> MNYEEVIKKYRGEENFDHAAYDWRLHSGVTPVKDQKNCGSAWAFSSIGSVESQYAIRKNKLITLSEQELVDCSFKNYGCNGGLINNAFEDMIELGGICPDGDY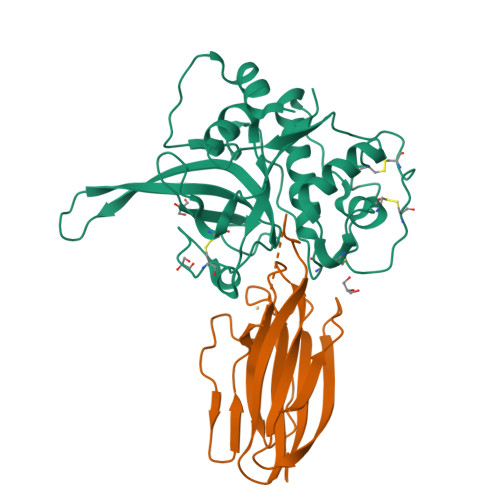PYVSDAPNLCNIDRCTEKYGIKNYLSVPDNKLKEALRFLGPISISVAVSDDFAFYKEGIFDGECGDQLNHAVMLVGFGMKEIVNPLTKKGEKHYYYIIKNSWGQQWGERGFINIETDESGLMRKCGLGTDAFIPLIE;> MGHHHHHHHHHHSSGHIEGRHMGDEKCGKSLKLGNISNQTNQETITQSLSVGEILCIDLEGNAGTGYLWVLLGIHKDEPIINPENFPTKLTKKSFFSEEISVTQPKKYKIDEHDSSKNVNREIESPEQKESDSKPKKPQMQLLGGPDRMRSVIKGHKPGKYYIVYSYYRPFSPTSGANTKIIYVTVQ> MTNLSDQTQQIVPFIRSLLMPTTGPASIPDDTLEKHTLRSETSTYNLTVGDTGSGLIVFFPGFPGSIVGAHYTLQGNGNYKFDQMLLTAQNLPASYNYCRLVSRSLTVRSSTLPGGVYALNGTINAVTFQGSLSELTDVSYNGLMSATANINDKIGNVLVGEGVTVLSLPTSYDLGYVRLGDPIPAIGLDPKMVATCDSSDRPRVYTITAADDYQFSSQYQPGGVTITLFSANIDAITSLSVGGELVFRTSVHGLVLGATIYLIGFDGTTVITRAVAANNGLTTGTDNLMPFNLVIPTNEITQPITSIKLEIVTSKSGGQAGDQMSWSARGSLAVTIHGGNYPGALRPVTLVAYERVATGSV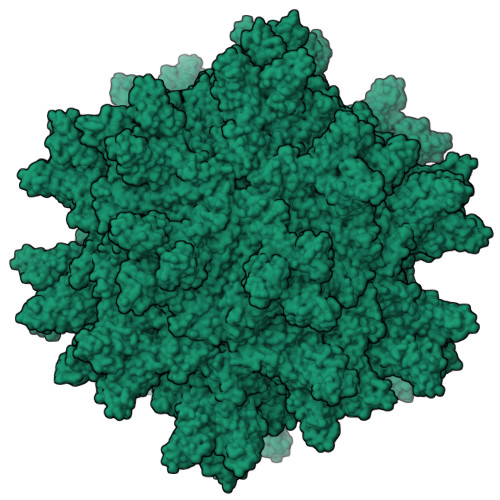VTVAGVSNFELIPNPELAKNLVTEYGRFDPGAMNYTKLILSERDRLGIKTVWPTREYTDFREYFMEVANLNSPLKIAGAFGFKDIIRAIR2'-deoxy-N-hydroxycytidine 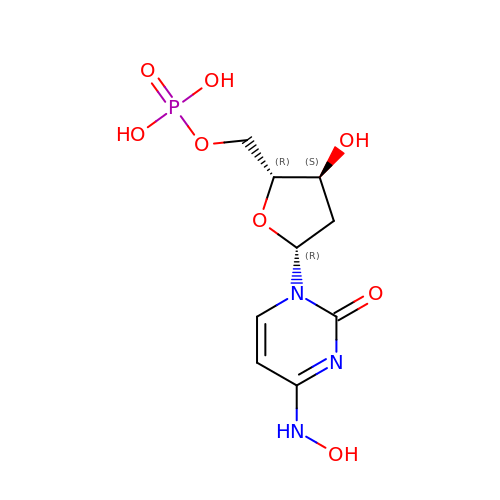5'-(dihydrogen phosphate) | C9 H14 N3 O8 P | YKOWBJJOJNGCAD-SHYZEUOFSA-N>[3x]GPLGSPLIGEIGPETYSDYMSAGIPLAYIFAET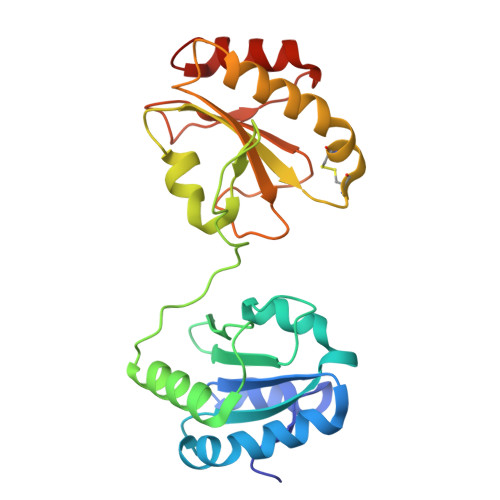AEERKELSDKLKPIAEAQRGVINFGTIDAKAFGAHAGNLNLKTDKFPAFAIQEVAKNQKFPFDQEKEITFEAIKAFVDDFVAGKIEPSIKSEPIPEKQEGPVTVVVAKNYNEIVLDDTKDVLIEFYAPWCGHCKALAPKYEELGALYAKSEFKDRVVIAKVDATANDVPDEIQGFPTIKLYPAGAKGQPVTYSGSRTVEDLIKFIAENGKYKAA> RPRLVWTPQLHKRFVDVVAHLGIKNAVPKTIMQLMNVEGLTRE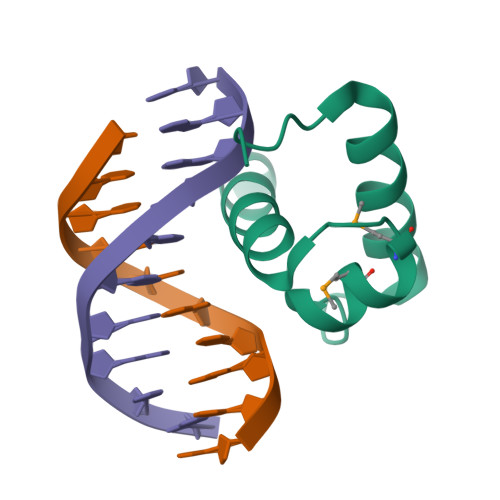NVASHLQKYRLYLK>[4x]MENFEIWVEKYRPRTLDEVVGQDEVIQRLKGYVERKNIPHLLFSGPPGTGKTATAIALARDLFGENWRDNFIEMNASDERGIDVVRH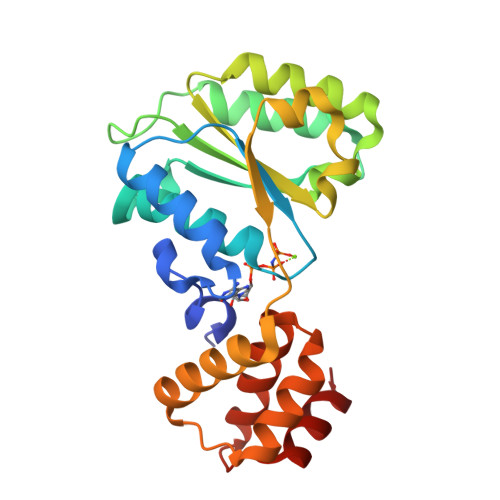KIKEFARTAPIGGAPFKIIFLDEADALTADAQAALRRTMEMYSKSCRFILSCNYVSRIIEPIQSRCAVFRFKPVPKEAMKKRLLEICEKEGVKITEDGLEALIYISGGDFRKAINALQGAAAIGEVVDADTIYQITATA The PotD-PotABC protein complex in Escherichia coli, belonging to the adenosine triphosphate–binding cassette transporter family, is a spermidine-preferential uptake system. In general, ATP binding, hydrolysis, and phosphate release trigger conformational changes in the transporter, leading to the uptake of extracellular polyamines. Here, we report structural details of the polyamine uptake system PotD-PotABC in various states.

Through three-dimensional (3D) classification, we successfully captured the ATP-bound state of the PotD-PotABC complex. In the translocation intermediate state (state 3), ATP binding to the PotA NBDs induces dimerization of NBDs and conformational changes of the coupling helices as well as the transmembrane helices (particularly TM3 to TM5), resulting in an outward-facing state of PotBC. The binding pockets of the two ATP molecules are symmetrically similar along the dimer interface, involving the signature Walker A and Walker B motifs from one PotA protomer and the LSGGQ motif from the other PotA protomer (PotA′). In contrast, the two lobes of PotD are observed to be in an “open” form in the translocation intermediate state, resulting in the formation of a cleft wide enough to provide a direct pathway for the Spd translocation. The periplasmic loop P3 (residues 198 to 228, between TM5 and TM6) in PotC protrudes into the PotD binding pocket and is designated as the “scoop loop. The K223 residue in the scoop loop forms extensive contacts with the residues W34, Y37, N213, W229, W255, and Y293 in PotD that participate in Spd binding in the pretranslocation state. Given its chemical structure similarity to Spd, it is likely that K223 mimics Spd interaction with PotD residues and prevents Spd from rebinding to PotD, thereby facilitating its translocation to the cytosol. We also observed a large cavity (with a volume of around 200 Å3) formed inside the PotBC. However, we could not observe any Spd molecules bound inside this cavity.

>[2x]MGQSKKLNKQPSSLSPLVQLAGIRKCFDGKEVIPQLDLTINNGEFLTLLGPSGCGKTTVLRLIAGLETVDSGRIMLDNEDITHVPAENRYVNTVFQSYALFPHMTVFENVAFGLRMQKTPAAEITPRVMEALRMVQLETFAQRKPHQLSGGQQQRVAIARAVVNKPRLLLLDQSLSALDYKLRKQMQNELKALQRKLGITFVFVTHDQEEALTMSDRIVVMRDGRIEQDGTPREIYEEPKNLFVAGFIGEINMFNATVIERLDEQRVRANVEGRECNIYVNFAVEPGQKLHVLLRPEDLRVEEINDDNHAEGLIGYVRERNYKGMTLESVVELENGKMVMVSEFFNEDDPDFDHSLDQKMAINWVESWEVVLADEEHK;> MKNTTSFQNVVIVTIVGWLVLFVFLPNLMIIGTSFLTRDDASFVKMVFTLDNYTRLLDPLYFEVLLHSLNMALIATLACLVLGYPFAWFLAKLPHKVRPLLLFLLIVPFWTNSLIRIYGLKIFLSTKGYLNEFLLWLGVIDTPIRIMFTPSAVIIGLVYILLPFMVMPLYSSIEKLDKPLLEAARDLGASKLQTFIRIIIPLTMPGIIAGCLLVMLPAMGLFYVSDLMGGAKNLLIGNVIKVQFLNIRDWPFGAATSITLTIVMGLMLLVYWRASRLLNKKVELE;> MIGRLLRGGFMTAIYAYLYIPIIILIVNSFNSSRFGINWQGFTTKWYSLLMNNDSLLQAAQHSLTMAVFSATFATLIGSLTAVALYRYRFRGKPFVSGMLFVVMMSPDIVMAISLLVLFMLLGIQLGFWSLLFSHITFCLPFVVVTVYSRLKGFDVRMLEAAKDLGASEFTILRKIILPLAMPAVAAGWVLSFTLSMDDVVVSSFVTGPSYEILPLKIYSMVKVGVSPEVNALATILLVLSLVMVIASQLIARDKTKGNTGDVK;> MKKWSRHLLAAGALALGMSAAHADDNNTLYFYNWTEYVPPGLLEQFTKETGIKVIYSTYESNETMYAKLKTYKDGAYDLVVPSTYYVDKMRKEGMIQKIDKSKLTNFSNLDPDMLNKPFDPNNDYSIPYIWGATAIGVNGDAVDPKSVTSWADLWKPEYKGSLLLTDDAREVFQMALRKLGYSGNTTDPKEIEAAYNELKKLMPNVAAFNSDNPANPYMEGEVNLGMIWNGSAFVARQAGTPIDVVWPKEGGIFWMDSLAIPANAKNKEGALKLINFLLRPDVAKQVAETIGYPTPNLAARKLLSPEVANDKTLYPDAETIKNGEWQNDVGAASSIYEEYYQKLKAGR> MDNVVLI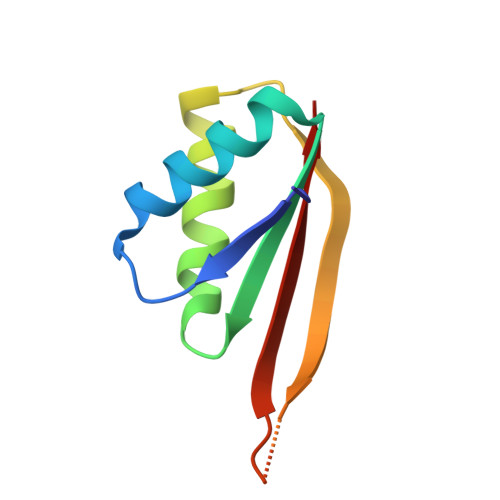GKKPVMNYVVAVLTQLTSNDEVIIKARGKAINKAVDVAEMIRNRFIKDIKIKKIEIGTDKVKNPDGREVNVSTIEIVLAK> MSLVLNDLLICCRQLEHDRATERKKEVEKFKRLIRDPETIKHLDRHSDSKQGKYLNWDAVFRFLQKYIQKETECLRIAKPNVSASTQASRQKKMQEISSLVKYFIKCANRRAPRLKCQELLNYIMDTVKDSSNGAIYGADCSNILLKDILSVRKYWCEISQQQWLELFSVYFRLYLKPSQDVHRVLVARIIHAVTKGCCSQTDGLNSKFLDFFSKAIQCARQEKSSSGLNHILAALTIFLKTLAVNFRIRVCELGDEILPTLLYIWTQHRLNDSLKEVIIELFQLQIYIHHPKGAKTQEKGAYESTKWRSILYNLYDLLVNEISHIGSRGKYSSGFRNIAVKENLIELMADICHQVFNEDTRSLEISQSYTTTQRESSDYSVPCKRKKIELGWEVIK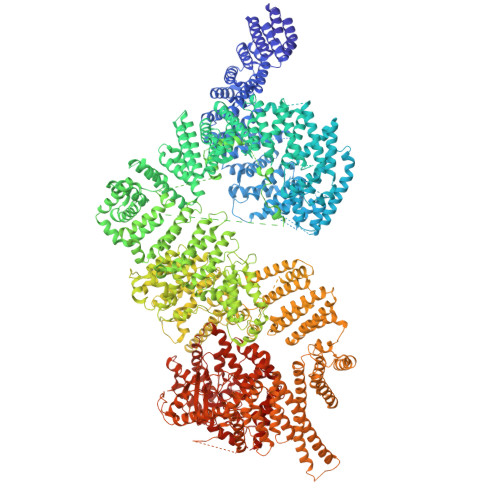DHLQKSQNDFDLVPWLQIATQLISKYPASLPNCELSPLLMILSQLLPQQRHGERTPYVLRCLTEVALCQDKRSNLESSQKSDLLKLWNKIWCITFRGISSEQIQAENFGLLGAIIQGSLVEVDREFWKLFTGSACRPSCPAVCCLTLALTTSIVPGTVKMGIEQNMCEVNRSFSLKESIMKWLLFYQLEGDLENSTEVPPILHSNFPHLVLEKILVSLTMKNCKAAMNFFQSVPECEHHQKDKEELSFSEVEELFLQTTFDKMDFLTIVRECGIEKHQSSIGFSVHQNLKESLDRCLLGLSEQLLNNYSSEITNSETLVRCSRLLVGVLGCYCYMGVIAEEEAYKSELFQKAKSLMQCAGESITLFKNKTNEEFRIGSLRNMMQLCTRCLSNCTKKSPNKIASGFFLRLLTSKLMNDIADICKSLASFIKKPFDRGEVESMEDDTNGNLMEVEDQSSMNLFNDYPDSSVSDANEPGESQSTIGAINPLAEEYLSKQDLLFLDMLKFLCLCVTTAQTNTVSFRAADIRRKLLMLIDSSTLEPTKSLHLHMYLMLLKELPGEEYPLPMEDVLELLKPLSNVCSLYRRDQDVCKTILNHVLHVVKNLGQSNMDSENTRDAQGQFLTVIGAFWHLTKERKYIFSVRMALVNCLKTLLEADPYSKWAILNVMGKDFPVNEVFTQFLADNHHQVRMLAAESINRLFQDTKGDSSRLLKALPLKLQQTAFENAYLKAQEGMREMSHSAENPETLDEIYNRKSVLLTLIAVVLSCSPICEKQALFALCKSVKENGLEPHLVKKVLEKVSETFGYRRLEDFMASHLDYLVLEWLNLQDTEYNLSSFPFILLNYTNIEDFYRSCYKVLIPHLVIRSHFDEVKSIANQIQEDWKSLLTDCFPKILVNILPYFAYEGTRDSGMAQQRETATKVYDMLKSENLLGKQIDHLFISNLPEIVVELLMTLHEPANSSASQSTDLCDFSGDLDPAPNPPHFPSHVIKATFAYISNCHKTKLKSILEILSKSPDSYQKILLAICEQAAETNNVYKKHRILKIYHLFVSLLLKDIKSGLGGAWAFVLRDVIYTLIHYINQRPSCIMDVSLRSFSLCCDLLSQVCQTAVTYCKDALENHLHVIVGTLIPLVYEQVEVQKQVLDLLKYLVIDNKDNENLYITIKLLDPFPDHVVFKDLRITQQKIKYSRGPFSLLEEINHFLSVSVYDALPLTRLEGLKDLRRQLELHKDQMVDIMRASQDNPQDGIMVKLVVNLLQLSKMAINHTGEKEVLEAVGSCLGEVGPIDFSTIAIQHSKDASYTKALKLFEDKELQWTFIMLTYLNNTLVEDCVKVRSAAVTCLKNILATKTGHSFWEIYKMTTDPMLAYLQPFRTSRKKFLEVPRFDKENPFEGLDDINLWIPLSENHDIWIKTLTCAFLDSGGTKCEILQLLKPMCEVKTDFCQTVLPYLIHDILLQDTNESWRNLLSTHVQGFFTSCLRHFSQTSRSTTPANLDSESEHFFRCCLDKKSQRTMLAVVDYMRRQKRPSSGTIFNDAFWLDLNYLEVAKVAQSCAAHFTALLYAEIYADKKSMDDQEKRSLAFEEGSQSTTISSLSEKSKEETGISLQDLLLEIYRSIGEPDSLYGCGGGKMLQPITRLRTYEHEAMWGKALVTYDLETAIPSSTRQAGIIQALQNLGLCHILSVYLKGLDYENKDWCPELEELHYQAAWRNMQWDHCTSVSKEVEGTSYHESLYNALQSLRDREFSTFYESLKYARVKEVEEMCKRSLESVYSLYPTLSRLQAIGELESIGELFSRSVTHRQLSEVYIKWQKHSQLLKDSDFSFQEPIMALRTVILEILMEKEMDNSQRECIKDILTKHLVELSILARTFKNTQLPERAIFQIKQYNSVSCGVSEWQLEEAQVFWAKKEQSLALSILKQMIKKLDASCAANNPSLKLTYTECLRVCGNWLAETCLENPAVIMQTYLEKAVEVAGNYDGESSDELRNGKMKAFLSLARFSDTQYQRIENYMKSSEFENKQALLKRAKEEVGLLREHKIQTNRYTVKVQRELELDELALRALKEDRKRFLCKAVENYINCLLSGEEHDMWVFRLCSLWLENSGVSEVNGMMKRDGMKIPTYKFLPLMYQLAARMGTKMMGGLGFHEVLNNLISRISMDHPHHTLFIILALANANRDEFLTKPEVARRSRITKNVPKQSSQLDEDRTEAANRIICTIRSRRPQMVRSVEALCDAYIILANLDATQWKTQRKGINIPADQPITKLKNLEDVVVPTMEIKVDHTGEYGNLVTIQSFKAEFRLAGGVNLPKIIDCVGSDGKERRQLVKGRDDLRQDAVMQQVFQMCNTLLQRNTETRKRKLTICTYKVVPLSQRSGVLEWCTGTVPIGEFLVNNEDGAHKRYRPNDFSAFQCQKKMMEVQKKSFEEKYEVFMDVCQNFQPVFRYFCMEKFLDPAIWFEKRLAYTRSVATSSIVGYILGLGDRHVQNILINEQSAELVHIDLGVAFEQGKILPTPETVPFRLTRDIVDGMGITGVEGVFRRCCEKTMEVMRNSQETLLTIVEVLLYDPLFDWTMNPLKALYLQQRPEDETELHPTLNADDQECKRNLSDIDQSFNKVAERVLMRLQEKLKGVEEGTVLSVGGQVNLLIQQAIDPKNLSRLFPGWKAWV>MDRKVQVLDFIKINPAGNITILIDNFDIYDKNIPKLSEEIMKETNLYAEQVGFIKDSHLQMMGGEFCGNASRAFASLLAFRDKDFSKQKNYNITCSGESKVLDVDVRNDGAKNKFLAKIKMPKFLSLEEINVDEYKLGLVRFSGINHFIFNIKENKETSFENIIDLVKKYLSNEEYSAFGIMFFDSDNLSMKPYVYVKEV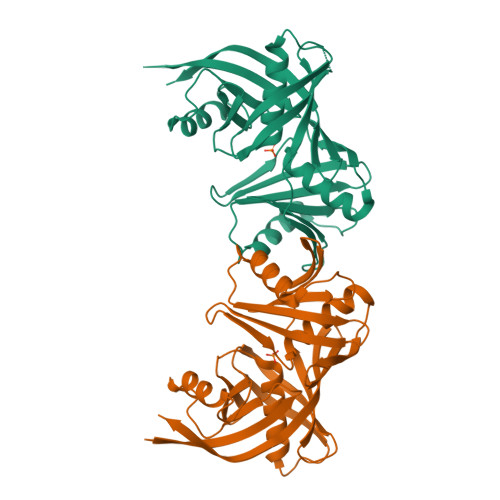GSGVYENSSASGTTALGYYLKKCKNLDRAKIVQPNGWLEYIIENDEMYIDGPVEIIAEGKIYIGKHHHHHH[4x]>[2x]GGGAEALELLEHCGVCRERLRPEREPRLLPCLHSACSACLGPAAPAAANSSGDGGAAGDGTVVDCPVCKQQCFSKDIVENYFMRDSGSKAATDAQDANQCCTSCEDNAPATSYCVECSEPLCETCVEAHQRVKYTKDHTVRSTGPAKSRDGERTVYCNVHKHEPLVLFCESCDTLTCRDCQLNAHKDHQYQFLEDAVRNQRKLLASLVKRLGDKHATLQKSTKEVRSSIRQVSDVQKRVQVDVKMAILQIMKELNKRGRVLVNDAQKVTEGQQERLERQHWTMTKIQKHQEHILRFASWALESDNNTALLLSKKLIYFQLHRALKMIVDPVEPHGEMKFQWDLNAWTKSAEAFGKIVAERPGTNSTGPAPMAPPRAPGPLSK;>[2x]SSDSEDVVSPNCSNTVQEKTFNKDTVIIVSEPSEDEESQGLPTMARRNDDISELEDLSELEDLKDAKLQTLKELFPQRSDNDLLKLIESTSTMDGAIAAALLMFGDAGGGPRKRKLSSSSEPYEEDEFNDDQSIKKTRLDHGEESNESAESSSNWEKQESIVLKLQKEFPNFDKQELREVLKEHEWMYTEALESLKVFAEDQDMQYVSQSEVPNGKEVSSRSQNYPKNATKTKLKQKFSMKAQNGFNKKRKKN

SMARCAD1 is a chromatin remodeler, a member of the SWI2/SNF2-like family of enzymes that couple ATP hydrolysis to repositioning, ejecting, or restructuring nucleosomes. KAP1 (also known as TRIM28 and TIF1β) is the major interaction partner of SMARCAD1, with the two proteins forming a tight complex (Okazaki et al., 2008, Rowbotham et al., 2011). The SMARCAD1-KAP1 interaction is direct and involves the first SMARCAD1 CUE domain (CUE1) and the RBCC domain of KAP1. Remarkably, CUE1, a canonical CUE domain, recognizes a cluster of exposed hydrophobic and surrounding charged/amphipathic residues on KAP1, which are presented in the context of a coiled-coil domain, not in a structure resembling ubiquitin.

We now crystallized the KAP1 RBCC domain (G53-K434) in complex with the SMARCAD1 CUE1,2 fragment (L94-N347). The structure was initially determined from a cubic crystal form to 5.5 Å resolution by single-wavelength anomalous diffraction, using the intrinsic anomalous signal of zinc ions. During model building and refinement, significant disordered sections of KAP1 were noted in the electron density maps. Electron densities for the first B-box domain could not be seen in the cubic form crystals (KAP1 RBCC-SMARCAD1 CUE 1,2 complex), nor could its zinc ions be located in anomalous difference maps, suggesting that this domain does not associate with the core, an interpretation supported by limited proteolysis experiments (data not shown). Similar to other TRIM family members (Goldstone et al., 2014, Sanchez et al., 2014, Weinert et al., 2015), the biological unit is a single, elongated dimer, which is symmetrical in the tetragonal crystal form (KAP1 RBCC ΔBBX1-SMARCAD1 CUE1,2 complex) but slightly asymmetric in the cubic crystal form (KAP1 RBCC-SMARCAD1 CUE 1,2 complex), suggesting that the coiled-coil domains may have a somewhat dynamic structure. In both cases, the dimer interface is extensive (∼5100 Å2) and formed primarily by the antiparallel association of the coiled-coil domains, with some contributions from the RING and second B-box domains. In both structures, electron density was only observed for a single CUE domain, which we conclude must be SMARCAD1 CUE1 based on our biochemical data. Our structural model shows a single SMARCAD1 CUE1 domain bound to each end of the KAP1 coiled-coil dimer.>RDLSYLLKIKELKEAKKEFEKIFIEEKL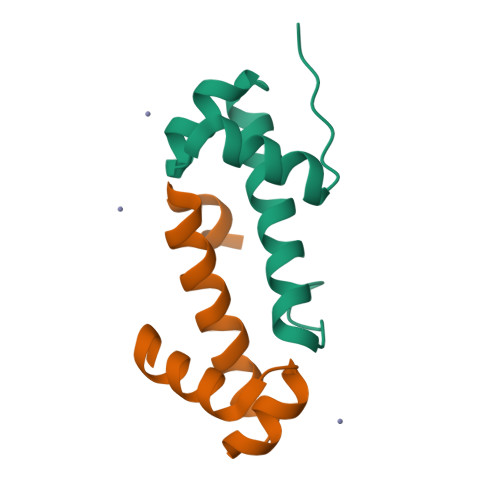REYDYDLKRTAEEIGIDLSNLYRKIKSLNIRVKSS[4x]>[2x]MFNRPILFDIVSRGS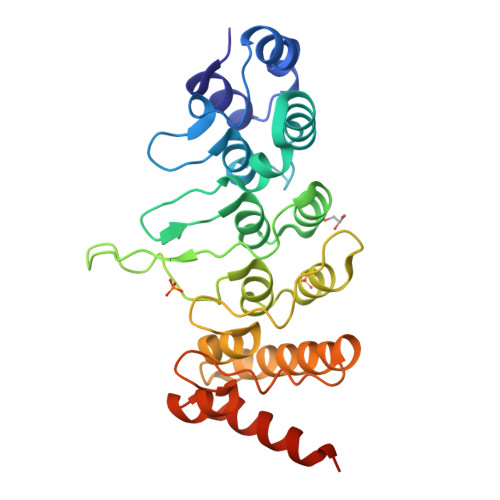TADLDGLLPFLLTHKKRLTDEEFREPSTGKTCLPKALLNLSNGRNDTIPVLLDIAERTGNMREFINSPFRDIYYRGQTALHIAIERRCKHYVELLVAQGADVHAQARGRFFQPKDEGGYFYFGELPLSLAACTNQPHIVNYLTENPHKKADMRRQDSRGNTVLHALVAIADNTRENTKFVTKMYDLLLLKCARLFPDSNLEAVLNNDGLSPLMMAAKTGKIGIFQHIIRREVTDEAAAHHHHHH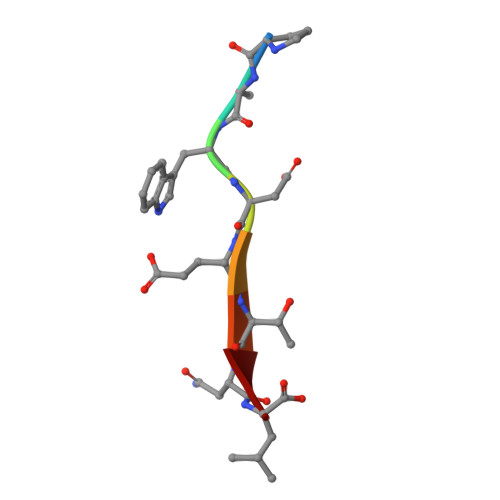> PAWDETNL> HHHHHHSSGLVPRGSHMASMLDMDDLATLDGQNWLNDQVINMYGELIMDAVPDKVHFFNSF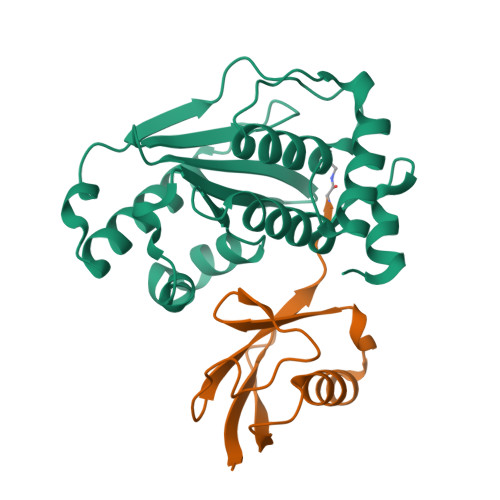FHRQLVTKGYNGVKRWTKKVDLFKKSLLLIPIHLEVHWSLITVTLSNRIISFYDSQGIHFKFCVENIRKYLLTEAREKNRPEFLQGWQTAVTKCIPQQKNDSDCGVFVLQYCKCLALEQPFQFSQEDMPRVRKRIYKELCECRLMD;> MGEYIKLKVIGQDSSEIHFKVKMTTHLKKLKESYCQRQGVPMNSLRFLFDGQRIADNHTPKELGMEEEDVIEVYQEQTGX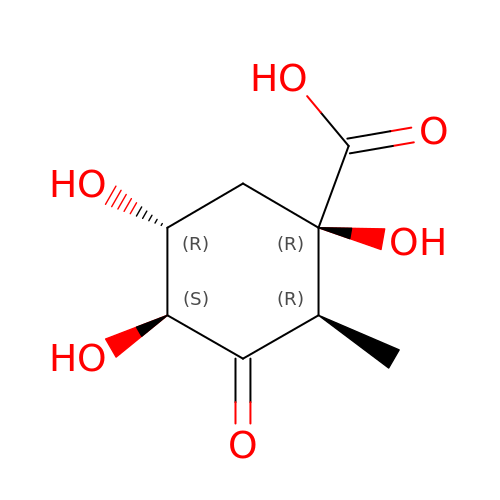(2R)-2-METHYL-3-DEHYDROQUINIC ACID | C8 H12 O6 | YHBCRPWBCJOXAZ-MIZGGHSWSA-N Human cytomegalovirus (HCMV), a ubiquitous beta-herpesvirus causing serious disease in immunocompromised individuals, encodes an abundant immediate-early protein termed IE1 that modulates innate immune mechanisms as well as other cellular processes. In addition to its effects on the innate immune system, IE1 is required to overcome the PML-NB-mediated intrinsic immunity that targets HCMV immediately upon infection. We present the first crystal structure for the evolutionary conserved core domain (IE1CORE) of primate cytomegalovirus IE1, which exhibits a novel, unusual fold. We show that this IE1CORE domain binds with high affinity to PML via the coiled-coil domain.

Crystallization trials with full-length hIE1 remained unsuccessful and, in case of the IE1CORE variants, yielded suitable crystals only for rhIE1CORE after chemical methylation of surface exposed lysine residues. The structure of rhIE1CORE was solved using experimental phases and refined to 2.3 Å resolution (Rwork = 19.73%, Rfree = 24.96%). The main chain of the model was traced between amino acids 41 and 393. RhIE1CORE adopts an elongated, femur-like shape with dimensions of 130×25×25 Å3. The structure can be divided into three distinct regions, namely an N-terminal head region (rhIE1: residues 62–118, 236–283; hIE1 residues 46–103, 221–267) and a C-terminal head region (rhIE1 residues 151–207, 315–393; hIE1 residues 136–192, 300–380) interconnected by a stalk region (rhIE1 residues 41–61, 119–150, 208–235, 284–314; hIE1 residues 27–45, 104–135, 193–220, 268–299). The stalk consists of an uncommon right-handed three-helix coiled-coil (α-helices H3, H6 and H9) with the N-terminal helix H1 added to one side of the three-helix bundle. RhIE1CORE forms a dimer with C2 point group symmetry in the crystal, and oligomerization of rhIE1 and hIE1 was confirmed both by gel filtration experiments and co-immunoprecipitation analyses (hIE1). RhIE1CORE dimerizes with both stalk regions juxtaposed in an antiparallel fashion. The main-chain conformation differs in the two monomers (Cα-RMSD for all helical segments  = 2.13 Å). This deviation originates from a pronounced kink that is observed in one of the two monomers and that causes a repositioning of the loop that interconnects helices H8 to H9 with a concomitant displacement of the N-terminal half of helix H9.

>GPLGSKQARKDMALQHAVDLLEKMLADEEKKLTEFNLGDPLFESANDDPIKTLEEIIQEGDDVVGAHQLVVTQIKLRVQRNRRLADEIIREQLTDIRKVFSDKFEKLEQGIQNSYLLLDKLKTPFQDMRCLFEVANEQFNDTPVPPQYKEKFMVCLKQIVQYAVNSSSKLEKFVMLKIKTKKDDIKDRVTYTCMKYLLMAMQGTGGPKAINNEEHAKLFFKQLSNYDDLTDANHDGLELIKKLDKEQKEVAFHVNNFTHLVTTLGMALYKEGHQKNDEAMLGMHTPITMLSDQVRVLILYLIDEIVHAIHTNSNQSNDELIDGLKPKVRIVINEFHATLMMGIDKMKFYSLNELREIVNDKINED[2x]>MNGERIIAFQGRPGAYSDLACRQARPGWTTLPCQTFAQTIAAVHDGRAELAMLACENSLAGRVPDIHALLPEAGLFIVGEHFQRVEHCLLGIPGSTLADARRIHTHPVAMAQVRGIITELGLDPVVEFDTAGAAEMVREWGRKEDVAVASALAAELNGLEILRRNVEDATHNTTRFYIASRRPATLPPPGPGFMTTLLFRVNNQPGALYKALGGLATAGVNMTRLESYMLEGSFSATQFLMDVEGHPEAPPLARALDELSFFSEQQEILGVYPASPFRRKP[2x]

GqqA strongly interfered with N-acyl-homoserine lactone (AHL) quorum sensing signals from Gram-negative bacteria and affected biofilm formation in its native host strain Komagataeibacter europaeus. ESI–MS–MS data showed unambiguously that GqqA hydrolyzes the amide bond of the acyl side-chain of AHL molecules, but not the lactone ring. Consistent with this observation the protein sequence does not carry a conserved Zn2+ binding motif, known to be essential for metal-dependent lactonases, but in fact harboring the typical periplasmatic binding protein domain (PBP domain), acting as catalytic domain. Structural data together with a phylogenetic analysis and the enzymatic characteristics implied that GqqA represents the first example of a till now unknown, third and novel subclass of acylases.

We report structural details for the native structure at 2.5 Å resolution and for a truncated GqqA structure at 1.7 Å. Crystals of GqqA and SeGqqA grew applying seeding within 3 days and belong to the space group P21 (GqqA) and P212121 (SeGqqA), respectively. Therefore, the crystal structure of SeGqqA was solved by single-wavelength anomalous diffraction (SAD) and refined to 1.7 Å resolution. The coordinates of the solved and refined structure of SeGqqA were suitable to solve the phase problem of native GqqA data by molecular replacement. The loss of this domain, which obviously appeared by proteolysis during the crystallization process of SeGqqA, resulted in crystals with different space group and cell dimensions, compared to GqqA. However, the obtained crystals were of higher quality. Due to the fold of the polypeptide chain in GqqA the missing domain for SeGqqA is located entirely at one side of the protein and has only a few interactions with the other domains. Superposition of the native GqqA on SeGqqA main chain atoms resulted in a Cα rms deviation of 0.76 Å, indicating that the missing domain of the SeGqqA structure did not change the overall fold of remaining two protein domains.> MSLSDSNDDRPFRPFQSQYRWPGVDLLAYKEEGSAPFRSVTRQVLFSGNGLTGELRYFEVGPGGHSTLERHQHAHGVMILKGRGHAMVGRAVSAVAPYDLVTIPGWSWHQFR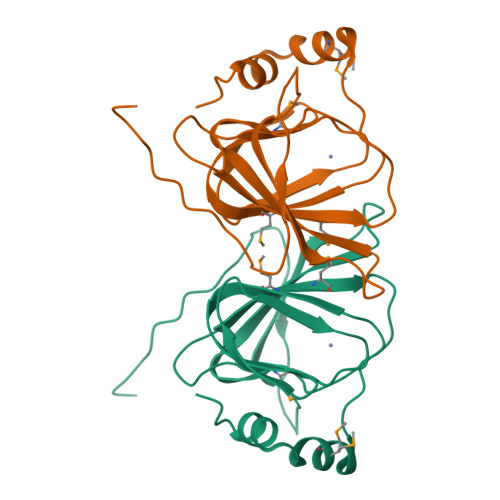APADEALGFLCMVNAERDKPQLPTEADLAMLRADDAVAAFLDGLAGEGHHHHHH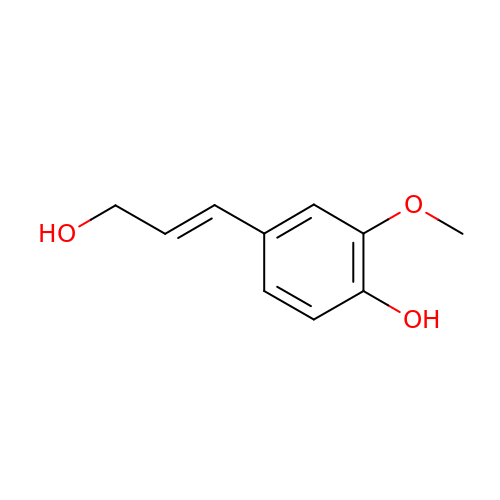4-[(1E)-3-hydroxyprop-1-en-1-yl]-2-methoxyphenol | C10 H12 O3 | JMFRWRFFLBVWSI-NSCUHMNNSA-N> GHMAQTDKHYFGTLLAQTSRAWRAELDRRLSHLGLSQARWLVLLHLARHRDSP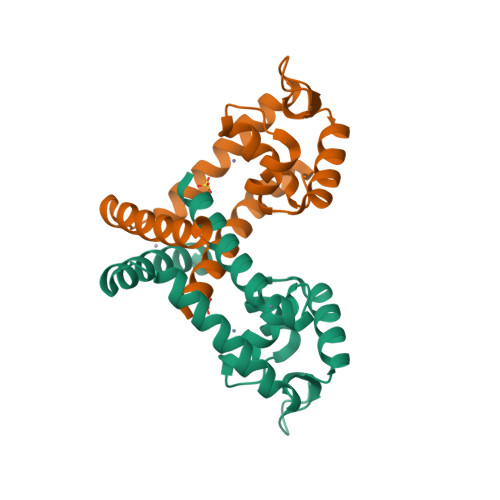TQRELAQSVGVEGPTLARLLDGLESQGLVRRLAVAEDRRAKHIVLTPKADVLIADIEAIAASVRNDVLTGIDESEQALCQQVLLRILANLENR> VKDLLKFLKAQTKTEEFDAIKIALASPDMIRSWSFGEVKKPETINYRTFKPERDGLFCARIFGPVKDYECLCGKYKRLKHRGVICEKCGVEVTQTKVRRERMGHIELASPTAHIWFLKSLPSRIGLLLDMPLRDIERVLYFESYVVIEGGMTNLERQQILTEEQYLDALEEFGDEFDAKMGAEAIQALLKSMDLEQECEQLREELNETNSETKRKKLTKRIKLLEAFVQSGNKPEWMILTVLPVLPPDLRPLVPLDGGRFATSDLNDLYRRVINRNNRLKRLLDLAAPDIIVRNEKRMLQEAVDALLDNGRRGRAITGSNKRPLKSLADMIKGKQGRFRQNLLGKRVDYSGRSVITVGPYLRLHQCGLPKKMALELFKPFIYGKLELRGLATTIKAAKKMVEREEAVVWDILDEVIREHPVLLNRAPTLHRLGIQAFEPVLIEGKAIQLHPLVCAAYNADFDGDQMAVHVPLTLEAQLEARALMMSTNNILSPANGEPIIVPSQDVVLGLYYMTRDCVNAKGEGMVLTGPKEAERLYRSGLASLHARVKVRITEYEKDA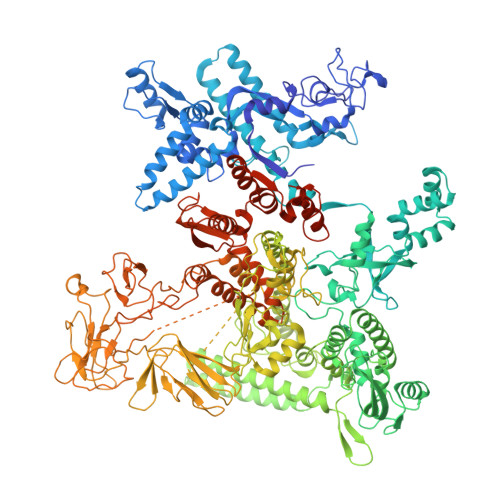NGELVAKTSLKDTTVGRAILWMIVPKGLPYSIVNQALGKKAISKMLNTCYRILGLKPTVIFADQIMYTGFAYAARSGASVGIDDMVIPEKKHEIISEAEAEVAEIQEQFQSGLVTAGERYNKVIDIWAAANDRVSKAMMDNLQTETVINRDGQEEKQVSFNSIYMMADSGARGSAAQIRQLAGMRGLMAKPDGSIIETPITANFREGLNVLQYFISTHGARKGLADTALKTANSGYLTRRLVDVAQDLVVTEDDCGTHEGIMMTPVIEGGDVKEPLRDRVLGRVTAEDVLKPGTADILVPRNTLLHEQWCDLLEENSVDAVKVRSVVSCDTDFGVCAHCYGRDLARGHIINKGEAIGVIAAQSIGEPGTQLTMRTFHIGGAASRAAAESSIQVKNKGSIKLSNVKSVVNSSGKLVITSRNTELKLIDEFGRTKESYKVPYGAVLAKGDGEQVAGGETVANWDPHTMPVITEVSGFVRFTDMIDGQTITRQTDELTGLSSLVVLDSAERTAGGKDLRPALKIVDAQGNDVLIPGTDMPAQYFLPGKAIVQLEDGVQISSGDTLARIPQESGGTKDITGGLPRVADLFEARRPKEPAILAEISGIVSFGKETKGKRRLVITPVDGSDPYEEMIPKWRQLNVFEGERVERGDVISDGPEAPHDILRLRGVHAVTRYIVNEVQDVYRLQGVKINDKHIEVIVRQMLRKATIVNAGSSDFLEGEQVEYSRVKIANRELEANGKVGATYSRDLLGITKASLATESFISAASFQETTRVLTEAAVAGKRDELRGLKENVIVGRLIPAGTGYAYHQDRMRRRAAGEAPAAPQVTAEDASASLAELLNAGLGGSDNELELEVLFQGPSSGHHHHHHHHHH>MGWCIFIYNLGQDADEGILWQMFGPFG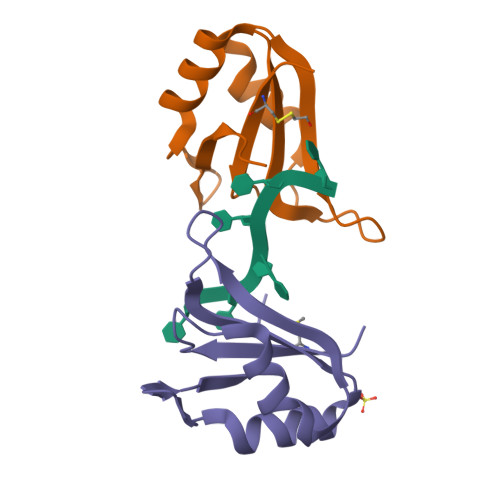AVTNVKVIRDFNTNKCKGFGFVTMTNYEEAAMAIASLNGYRLGDKILQVSFKTNKSHK[3x]>MQSTSNHLWLLSDILGQGATANVFRGRHKKTGDLFAIKVFNNISFLRPVDVQMREFEVLKKLNHKNIVKLFAIEEETTTRHKVLIMEFCPCGSLYTVLEEPSNAYGLPESEFLIVLRDVVGGMNHLRENGIVHRNIKPGNIMRVIGEDGQSVYKLTDFGAARELEDDEQFVSLYGTEEYLHPDMYERAVLRKDHQKKYGATVDLWSIGVTFYHAATGSLPFRPFEGPRRNKEVMYKIITGKPSGAISGVQKAENGPIDWSGDMPVSCSLSRGLQVLLTPVLANILEADQEKCWGFDQFFAETSDILHRMVIHVFSLQQMTAHKIYIHSYNTATIFHELVYKQTKIISSNQELIYEGRRLVLEPGRLAQHFPKTTEENPIFVVSREPLNTIGLIYEKISLPKVHPRYDLDGDASMAKAITGVVCYACRIASTLLLYQELMRKGIRWLIELIKDDYNETVHKKTEVVITLDFCIRNIEKTVKVYEKLMKINLEAAELGEISDIHTKLLRLSSSQGTIETSLQDIDSRLSPGGSLADAWAHQEGTHPKDRNVEKLQVLLNCMTEIYYQFKKDKAERRLAYNEEQIHKFDKQKLYYHATKAMTHFTDECVKKYEAFLNKSEEWIRKMLHLRKQLLSLTNQCFDIEEEVSKYQEYTNELQETLPQKMFTASSGIKHTMTPIYPSSNTL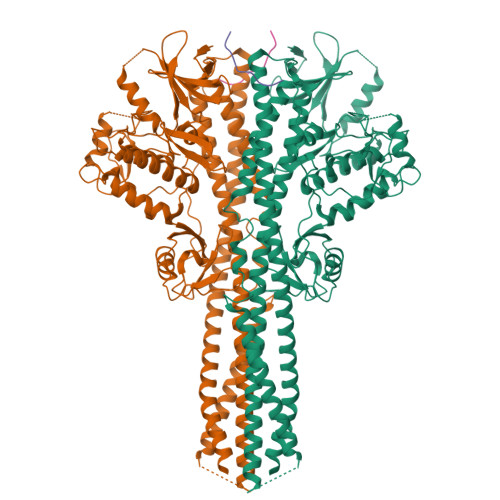VEMTLGMKKLKEEMEGVVKELAENNHILERFGSLTMDGGLRNVDCLGIHRPDYKDDDDK[2x];>MPQDPSTRSSPARLLIPEPRAGRARHAACVLLAVCFVVLFLSGEPLAPIIRSVCTQLAALQLGVLLKGCCCLAEEIFHLHSRHHGSLWQVLCSCFPPRWYLALLLVGGSAYLDPPEDNGHSPRLALTLSCLCQLLVLALGLQKLSAVEVSELTESSKKNVAHGLAWSYYIGYLKVVLPRLKECMEELSRTNPMLRAHRDTWKLHILVPLGCDIWDDLEKADSNIQYLADLPETILTRAGIKRRVYKHSLYVIRDKDNKLRPCVLEFASPLQTLCAMSQDDCAAFSREQRLEQARLFYRSLRDILGSSKECAGLYRLIAYEEPAEPESHFLSGLILWHLQQQQREEYMVQEELPLGTSSVELSLQVSSSDLPQPLRSDCPGIHRPDYKDDDDK[2x]4-AMINO-2-HYDROXYBUTANOIC ACID | C4 H9 N O3 | 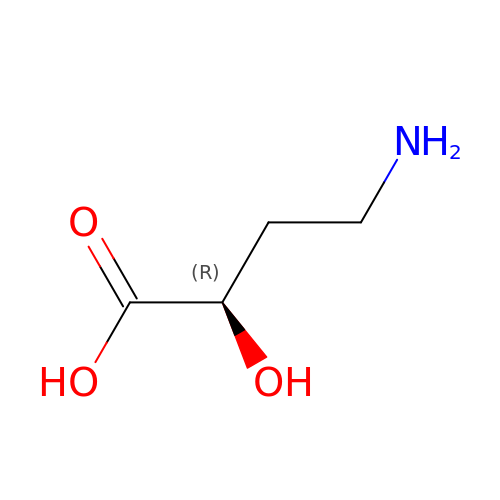IVUOMFWNDGNLBJ-GSVOUGTGSA-N>GMDPKHGNLFADVPVGAPDEIFQPLLERKGLKIERIISNGQASPPGFWYDSPQDEWVMVVSGSAGI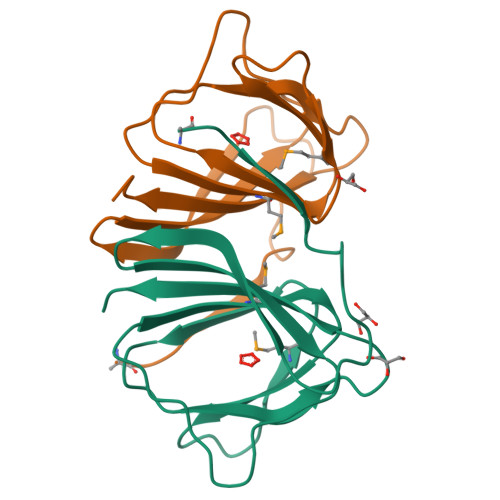ECEGDTAPRVMRPGDWLHVPAHCRHRVAWTDGGEPTVWLAVHCDAA[4x]>[2x]FKTIKSDEIFAAAQKLMPGGVSS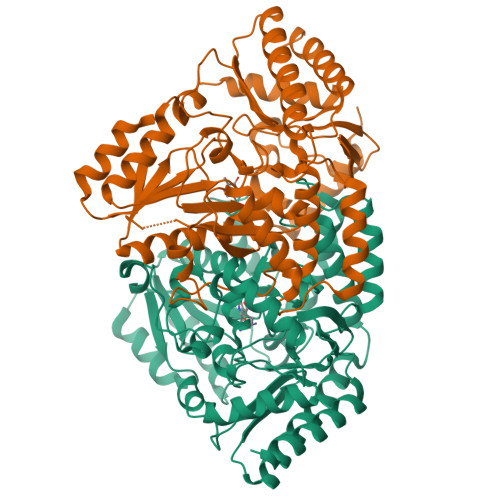PVRAFKSVGGQPIVFDRVKDAYAWDVDGNRYIDYVGTWGPAICGHAHPEVIEALKVAMEKGTSFGAPCALENVLAEMVNDAVPSIEMVRFVNSGTEACMAVLRIMRAYTGRDKIIKFEGCYHGHADMFLVKAGSGVATLGLPSSPGVPKKTTANTLTTPYNDLEAVKALFAENPGEIAGVILEPIVGNSGFIVPDAGFLEGLREITLEHDALLVFDEVMTGFRIAYGGVQEKFGVTPDLTTLGKIIGGGLPVGAYGGKREIMQLVAPAGPMYQAGTLSGNPLAMTAGIKTLELLRQPGTYEYLDQITKRLSDGLLAIAQETGHAACGGQVSGMFGFFFTEGPVHNYEDAKKSDLQKFSRFHRGMLEQGIYLAPSQFEAGFTSLAHTEEDIDATLAAARTVMSAL>MALSKVKLNDTLNKDQLLSSSKYTIQRSTGDSIDTPNYDVQKHINKLCGMLLITEDANHKFTGLIGMLYAMSRLGREDTIKILRDAGYHVKANGVDVTTHRQDINGKEMKFEVLTLASLTTEIQINIEIESRKSYKKMLKEMGEVAPEYRHDSPDCGMIILCIAALVITKLAAGDRSGLTAVIRRANNVLKNEMKRYKGLLPKDIANSFYEVFEKHPHFIDVFVHFGIAQSSTRGGSRVEGIFAGLFMNAYGAGQVMLRWGVLAKSVKNIMLGHASVQAEMEQVVEVYEYAQKLGGEAGFYHILNNPKASLLSLTQFPHFSSVVLGNAAGLGIMGEYRGTPR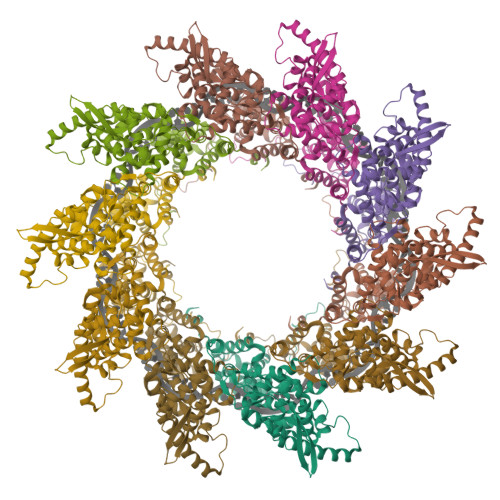NQDLYDAAKAYAEQLKENGVINYSVLDLTAEEL[10x]>[2x]MSLSKKRKLESGDSGGA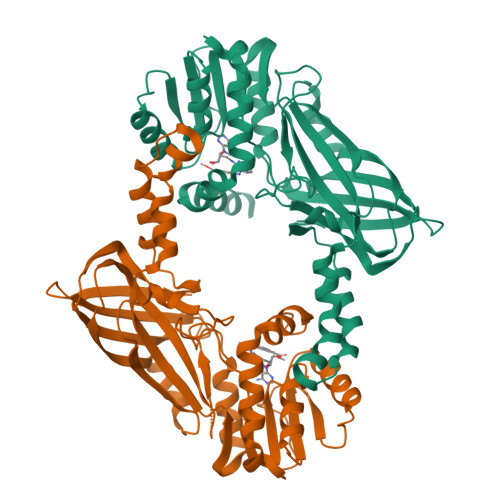GAGGEGAEEENGGEQEAAPPRPRRTKSERDQLYYECYSDVSVHEEMIADQVRTEAYRLGILKNWAALRGKTVLDVGAGTGILSIFCAQAGARRVYAVEASAIWQQAREVVRLNGLEDRVHVLPGPVETVELPERVDAIVSEWMGYGLLHESMLSSVLHARTKWLKEGGLLLPASAELFVAPISDQMLEWRLGFWSQVKQHYGVDMSCMESFATRCLMGHSEIVVQDLSGEDVLARPQRFAQLELARAGLEQELEAGVGGRFRCSCYGSAPLHGFAVWFQVTFPGGDSEKPLVLSTSPLHPATHWKQALLYLNEPVPVEQDTDISGEITLLPSPDNPRRLRILLRYKVGDHEEKTKDFAMEDGSENLYFQ(3aS,4S,6aR)-4-(5-{1-[(3-fluorophenyl)methyl]-1H-1,2,3-triazol-4-yl}pentyl)tetrahydro-1H-thieno[3,4-d]imidazol-2(3H)-one | C19 H24 F N5 O S | 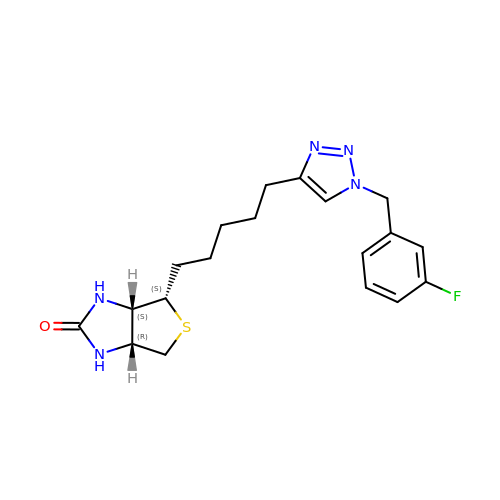RJRZSEAZACQQJO-BZSNNMDCSA-N The neuraminidase inhibitors (NAIs) oseltamivir and zanamivir are the antiviral agents available in France to treat influenza A or B virus infections. The NA active site includes catalytic residues (R118, D151, R152, R224, E276, R292, R371, and Y406; N2 numbering) that interact directly with the sialic acid substrate and framework residues (E119, R156, W178, S179, D/N198, I222, E227, H274, E277, N294, and E425; N2 numbering) that stabilize the active site. NAs are divided into 3 phylogenic groups: influenza B viruses, group 1 (N1, N4, N5, and N8), and group 2 (N2, N3, N6, N7, and N9) from influenza A viruses. I221 (B NA numbering), I222 (N2 numbering), and I223 (N1 numbering) amino acids are highly conserved framework residues in NAs of influenza viruses.

We are the first to report influenza B viruses, isolated from an immunocompromised patient after prolonged oseltamivir treatment, with good fitness carrying a novel I221L substitution (B numbering) in NA that confers high-level resistance to oseltamivir. We used X-ray crystallography to understand the structural basis of resistance to oseltamivir conferred by NA carrying the I221L substitution. Crystals of the NA-I221L protein in complex with both inhibitors diffracted to high resolution, showing clearly defined density for bound oseltamivir and zanamivir. Consistent with lower levels of inhibition of the I221L mutant virus by zanamivir, no marked changes in the conformation of zanamivir were seen. Viruses isolated from an NPA collected on D34 and a nasal swab specimen collected on D40 were highly resistant to oseltamivir (IC50, 1515 and 1776 nM, respectively) and showed reduced inhibition by zanamivir (IC50, 24.3 and 27.3 nM, respectively), compared with the first wild-type isolate. The Km revealed that the I221L NA variant had a 1.9 times lower affinity for the MUNANA substrate, and the Ki values for oseltamivir carboxylate and zanamivir showed affinities that were around 84 and 51 times lower, respectively, than that for wild-type NA.

>[8x]MLPSTIQTLTLFLTSGGVLLSLYVSALLSYLLYSDILLKFSPTEITAPTMSLDCANASNVQAVNRSATKGVTFLLPEPEWTYPRLSCPGSTFQKALLISPHRFGETKGNSAPLIIREPFIACGPNECKHFALTHYAAQPGGYYNGTRGDRNKLRHLISVKLGKIPTVENSIFHMAAWSGSACHDGKEWTYIGVDGPDNDALLKVKYGEAYTDTYHSYANKLLRTQESACNCIGGNCYLMITDGSASGVSECRFLKIREGRIIKEIFPTGRVKHTEECTCGFASNKTIECACRDNSYTAKRPFVKLNVETDTAEIRLMCTDTYLDTPRPDDGSITGPCESNGDKGSGGIKGGFVHQRMESKIGRWYSRTMSKTERMGMGLYVKYDGDPWADSDALAFSGVMVSMKEPGWYSFGFEIKDKECDVPCIGIEMVHDGGKETWHSAATAIYCLMGSGQLLWDTVTGVDMAL>GPGSMGRVQDKVVLVTGGARGQGRSHAVKLAEEGADIILFDICHDIETNEYPLATSRDLEEAGLEVEKTGRKAYTAEVDVRDRAAVSRELANAVAEFGKLDVVVANAGICPLGAHLPVQAFADAFDVDFVGVINTVHAALPYLTSGASIITTGSVAGLIAAAQPPGAGGPQGPGGAGY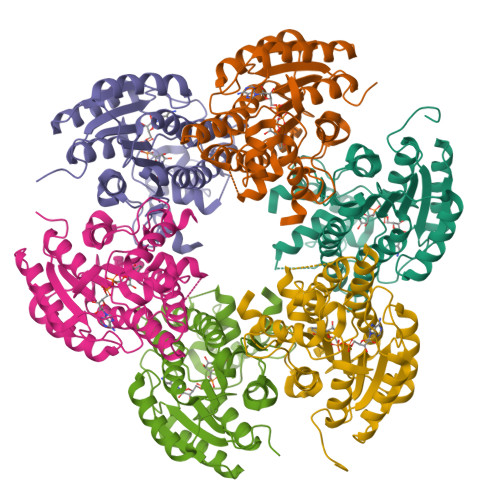SYAKQLVDSYTLQLAAQLAPQSIRANVIHPTNVNTDMLNSAPMYRQFRPDLEAPSRADALLAFPAMQAMPTPYVEASDISNAVCFLASDESRYVTGLQFKVDAGAMLKF[6x]RCs are classified as type I or type II, depending on whether their terminal electron acceptors are in the form of iron–sulfur clusters or quinones. Among these anoxygenic photosynthetic bacteria, green sulfur bacteria such as Chlorobium tepidum (C. tepidum, phylum Chlorobi), heliobacteria such as Heliomicrobium modesticaldum (H. modesticaldum, phylum Firmicutes), some Chloroflexi such as Candidatus Chlorohelix allophototropha (phylum Chloroflexi)8 and Acidobacteria such as Chloracidobacterium thermophilum (C. thermophilum, phylum Acidobacteria)9 have homodimeric type I RCs. Here, we solve the structures of the RC from C. thermophilum (CabRC) by single-particle cryo-electron microscopy (cryo-EM) at resolutions of 2.61 Å for a larger form (termed CabRCL) and 2.22 Å for a smaller form (termed CabRCS). In both structures, two distinctive c-type cytochromes (Cyts c) are tightly bound, making the anticipated type I RC structures with cytochromes bound be solved.

The CabRCL form (2.61 Å resolution) possessed two additional extrinsic subunits on the cytoplasmic side, PscB (an electron acceptor protein containing two Fe4S4 clusters corresponding to PscB in the GsbRC) and PscZ (a newly identified subunit whose binding position is analogous to that of PscD in the GsbRC), forming a larger structure with dimensions of ~130 Å × 120 Å × 100 Å. Except for the extra PscB and PscZ, CabRCL was almost the same as CabRCS. As CabRCL binds electron donor and acceptor proteins, we describe the characteristics of CabRC based primarily on CabRCL. CabRCL contained numerous cofactors, including 16 BChls a, 2 Zn-BChls a′, 10 Chls a, 2 lycopenes, 12 lipids [2 phosphatidyl-ethanolamines (PE), 6 phosphatidyl-N-methylethanolamines (PME) and 4 diacylglycerylhydroxymethyl-N,N,N-trimethylalanines (DGTA)], 3 Fe4S4 clusters (FX, FA, and FB), 2 heme groups (Heme1 and Heme2), 2 Ca2+ ions, 6 water molecules and 32 unknown molecules, in addition to the 12 protein subunits and two UPPs. PscZ, consisting of 60 amino acids (M1–L60) and forming a two-helix structure, resided at the cytoplasmic side and connected to PscB through hydrophobic interactions, hydrogen bonds, and salt bridges. Further analysis revealed that the PscB/CabRC binds to the surface of its RC core mainly through the weak electrostatic interactions between the negatively charged patch on the PscB side and the positively charged patch on the CabRC core side, as well as one weak hydrogen bond between D91/PscB and K701/PscA-2, which is consistent with the fact that the PscB and PscZ subunits in the CabRC are easily removed during purification.

>[2x]ANGVKRWYQKLELPMPPERIFGAHMMLIGGLACLIGTYFFASMTMWNDGYVNLTLRPRLISLGIYDPYDTEQIQRVWLPLIGEFSTSKLPFFGQYPLTMTDFRLFGWGCFHIGLGLWLVYAGAAHYYGARGGATIGEIFWLLPYVPGLKGLCQIKWFTPEGPWYKVGLPWGSFANTPWPILRRTYADALSPHTIYIGLLFFIWGFVLWFVLDKPPVPLQPAQVMTPNGLMPLEQAPFPYGWFDPYLNQVMHPMNTINGETTMCFVWGVLFVALGAYWWYRPPRSINITHLEDTKAVFHVHLTAIGYVSFALAIVGFLALRNHPSYLMLNDMNVIIYGKKIVNPGRMIHNMITFNHVQVGLLYVAAGVFHGGQYLHGLNISGAYKQARSKFITWFQNPDLQTKIVGTTMFVSFVTVVFGYGMICWNTGAELDLNFGIYQFRSFRAIQMDGEAGNIGYRVFRPKNPWDPTAGGDWVKNPDGTAKLVKARNLQVGDRILNEELGIGSSPTYSFTTIEEINYKPEWGQPKLYAVQWGSWTHFLRKVNPLFWVDKGIWYLQNQKTFEATRKADEAYLAAHLKAVSLLNQIDDAQTEEAKQKAQAELDKFRPELEKAHANMLEWNERLASTPAVLYSNLRDQHRDGEINDAIFFWLMIGGWLFGFIPLLRIAFHNYQSPWYRDFEWRKQSPDFPCIGPVKGGTCGVSIQDQLWFCILFSIKPLSAIAWYLDGGWIATMMARGNEAYYLTHNISHTGGVFLYMWNETTWIWTDNHLTAMLLLGHLIWFVSFALWFKDRGSRAEGGDIQSRWVRLMGKRLGIKTLQEVRFPVSNLATAKLWGTVFFYTGTFVLVFLYFADGFFQNR;> QIYTIIEELCIGCGFCTDECPPKVNAILPRDVEAVLDGGETYWIDQTRCISCSLCFVAGTCPTDAVVFTEGGVSRT;> LLVGGCFVGSRDPNETRYPKAPMPLQNQTSTLKTAEEIRRESVAQNTPGAREAAALRDRVTPLNLQQVNEQDVAGNDPLGSPARVVLDEGEMYRDPVEIYREGRALFQNNCVGCHGHNGCGNVPRSTNFTDPGWQENNSDGGIYSSIYNGKGIGNGGGAMPAYYNQLSPQQIRYLVAYLRAFKGRQCNGLPTLSDVERMVAERQ;> MARTPEEIVKRYKEANIWLRHWKQQIGLAKDEEQREMFTQYYEERVQEIAALEEPYRAALKILNQQESQR;>MTAILLACLFVLGGYAALWGIIKFVVANTKDIAAN[2x];>[2x]MWNVVGQIISVLCFFILTVGTLFGIVYVSHLLSRG;>[2x]DISKVAWAWFGVLLAICLIGAFGNYVPKLFVKMLMFLN;> VMATGCFVGARNASEPRLGSSSIAASRTAPAYLREAQVLYEGSTDGLPKDTPADEIAHYKAMLAELQTRNYAACAGCHQVNGGGNKAINATNFQDAGWQANNSSPGMVTSIVNGKGKVMPAYKDKLTLQQINYLVEYIRRFEKKR>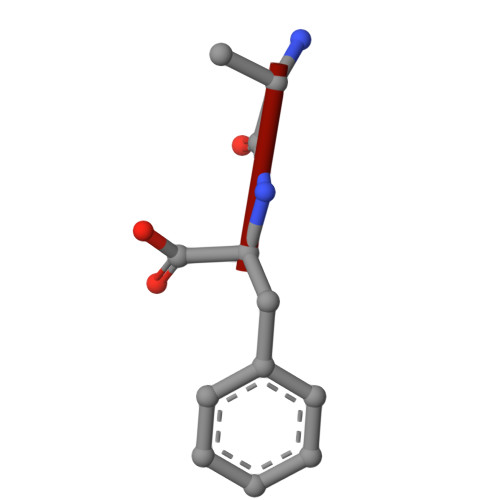 AF> MIDTWLAQWGLRLPSSNDATLRLQPAEGPELVMERLEGGWLFVVELGLVPSGLPLGVILQLLQVNSPFSSLAPVKLAADDAGRLVLWAEARDGVDDVDALNRLHDRLREGHSRLVPLLEPTGEL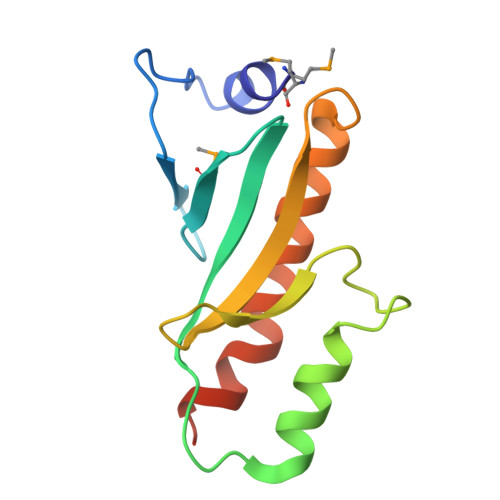VPA> MLRVLVGAVLPAMLLAAPPPINKLALFPDKSAWCEAKNITQIVGHSGCEAKSIQ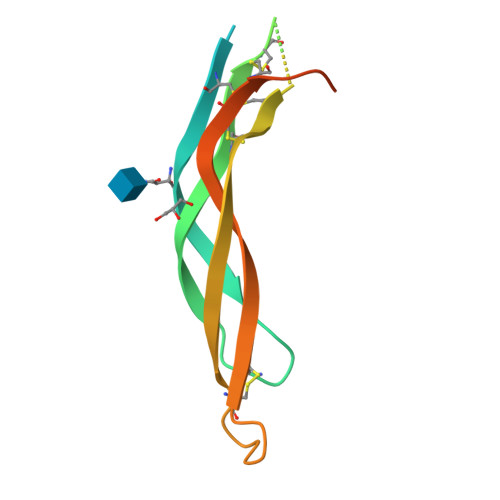NRACLGQCFSYSVPNTFPQSTESLVHCDSCMPAQSMWEIVTLECPGHEEVPRVDKLVEKILHCSCQACGKEPSHEGLSVYVQGED> QDNSRYTHFLTQHY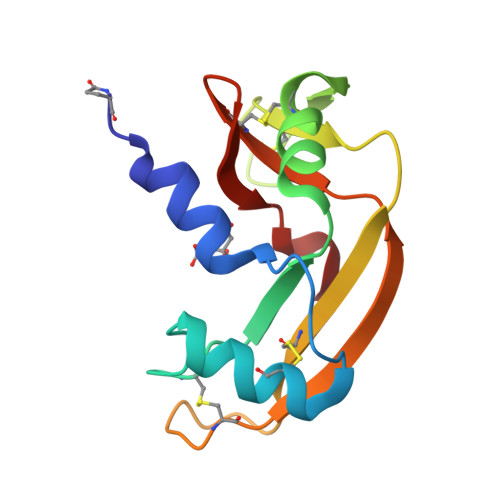DAKPQGRDDRYCESIMRRRGLTSPCKDINTFIHGNKRSIKAICSQKNVACKNGQTNCYISKSSFQVTTCKLHGGSPWPPCQYRATAGFRNVVVACENGLPVHLDQSIFR> APSDLSALIPRATFDQMLKHRNDGACPARGFYTYDAFIAAARAFPSFGNTGDTATRKREIAAFLGQTSHETTGGWPSAPDGPYAWGYCFVREQNPSAYCSPTPQFPCASGQQYYGRGPIQISWNYNYGQCGNAIGVDLINNPDLVATDPVVSFKSAIWFWMTPQSPKPSSHDVITSQWTPSAADVAA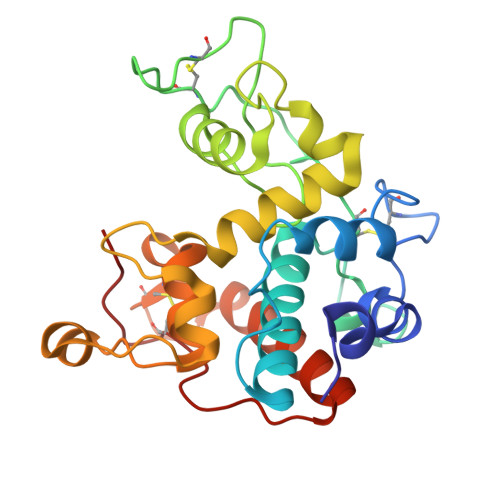GKLPGYGTVTNIINGGLECGRGQDSRVEDRIGFFKQYCDLFGVGYGNNLDCYSQAPFG> RRASLHRFLEKRKDRVTSKA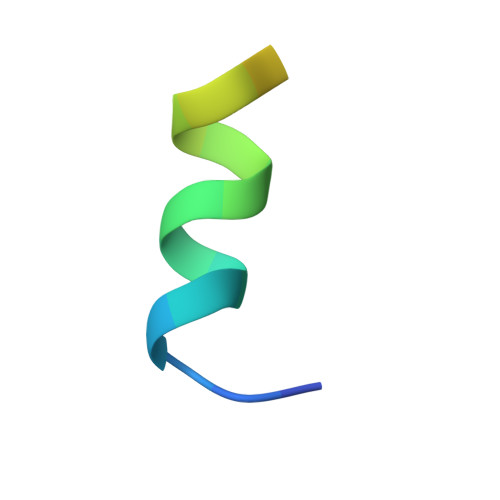PY> CAGCAGCCTGAATA;> GGCTGC;> GCGAGTATTCACCGGCTCCGCGGTTTTCCGCGGCTCGCAGCCGGACAGCG;> TGCGCTGT

A well‐studied, DNA tensegrity triangle crystal were explored as a crystal scaffold to regularly arrange DNA T‐junction motifs in 3D space. T‐junction is a T‐shaped, structural motif designed by Satoshi Murata and Hamada Shogo. It is formed by hybridization between a single‐stranded DNA (ssDNA) sticky end (black) of a DNA duplex and a ssDNA bulge loop of another DNA duplex (green). For structural characterization, a T‐junction is incorporated at the center helical domain of each component duplex of the triangle, resulting in a modified, T‐junction triangle (ΔT) motif. The T‐junction triangle is named as ΔTm‐n. ΔT stands for T‐junction‐containing triangle; numbers m and n indicate the distance (in base pairs, bps) between the hairpin and the left corner of the triangle and the length (in bps) of the side duplex arm (C‐arm), respectively.

The crystals of all the ΔT variants were studied by X‐ray crystallography. They all shared R3 rhombohedral lattices with the same unit cell dimensions: a = b = c ∼100 Å and α = β = γ = 112 – 114°. The data matched with the parameters of conventional 3‐turn tensegrity triangle crystals within 3% error; indicating that the overall DNA triangle frameworks remained the same for all ΔT variants. Indeed, for all ΔT variants, extra densities (colored green) could clearly be identified (e for ΔT7‐6, S3d and S3e for ΔT6‐6, S4d and S4e for ΔT6‐11, S5d and S5e for ΔT7‐11, S6d and S6e for ΔT8‐6, S7d and S7e for ΔT8‐11). In ΔT6‐6 and ΔT6‐11, the extra densities were directly below the triangle planes. For crystals with the same C‐arm positions, the orientations and the locations of the extra C‐arms were almost identical. When the C‐arm position was the same, the triangles could pretty much completely overlap with each other, ΔT6‐6/ΔT6‐11, ΔT7‐6/ΔT7‐11, and ΔT8‐6/ΔT8‐11, except the C‐arm lengths. More interesting was superimposing the triangles with C‐arms of the same length but different C‐arm positions, ΔT6‐6/ΔT7‐6/ΔT8‐6/ and ΔT6‐11/ΔT7‐11/ΔT8‐11/. By looking along the triangle edge duplex, the C‐arms rotated stepwise by 28°–54° (rotating angles from ΔT6‐6 to ΔT7‐6 to ΔT8‐6 are 28° and 54°, respectively; rotating angles from ΔT6‐11 to ΔT7‐11 to ΔT8‐11 are 43° and 37°, respectively), consistent with the twist of 34°/bp for B‐DNA duplex.One especially common junction element is the kink-turn (k-turn). k-turns are elements in double-stranded RNA that introduce a tight kink into the helical axis, with an included angle close to 50°. A standard k-turn comprises a three-nucleotide bulge followed by successive G•A and A•G trans G(sugar edge)•A(Hoogsteen edge) basepairs. k-turns are commonly-occurring motifs that introduce sharp kinks into duplex RNA, thereby facilitating tertiary contacts. Both the folding and conformation of k-turns are determined by their local sequence. k-turns fall into two conformational classes, called N3 and N1, that differ in the pattern of hydrogen bonding in the core. We show here that this is determined by the basepair adjacent to the critical G•A pairs.

We therefore decided to extend the study with a systematic structural analysis of HmKt-7 as a function of the 3b,3n sequence. This was performed in the constant environment of the SAM-I riboswitch, modified by replacing its natural k-turn by HmKt-7 with different 3b,3n sequences. In this way we could observe the effect of changing the 3b,3n sequence alone in an otherwise completely unchanged RNA molecule. There is a tendency for 3b = purine to result in an N3 structure, but the generality is broken by the N1 structure adopted by the 3b,3n = G•G Kt-7 variant. Moreover, the structures of the HmKt-7 variants inserted into the SAM-I riboswitch demonstrate that changing the 3b,3n sequence is sufficient to switch the equilibrium conformation of the k-turn.

> GGCUUAUCAAGAGAGGGUGAGCGACUGGCGCGAAGAGCCCCGGCAACCAGAAAUGGUGCCAAUUCCUGCAGCGGAAACGUUGAAAGAUGAGCCG> GAMGSAVSESQLKKMVSKYKYRDLTVRETVNVITLYKDLKPVLDSYGTGSRELMNLTGTIPVPYRGNTYNIPICLWLLDTYPYNPPICF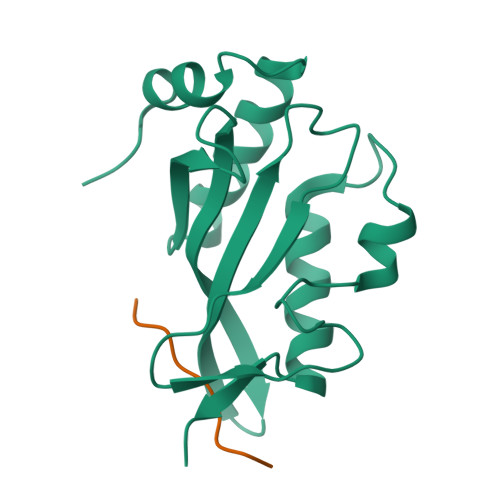VKPTSSMTIKTGKHVDANGKIYLPYLHEWKHPQSDLLGLIQVMIVVFGDEPPVFSRP;> PEPTAPPEE> MAHHHHHHMKFAFVFPGQGSQSVGMLNAFADVAVVRETLDEASDALGQDIGKLIADGPADELNLTTNTQPVMLTAAYACYRAWQQAGGAQPSIVAGHSLGEYTALVAAGAIAFRDALPLVRFRAQAMQTAVPVGVGGMAAILGLDDDTVRAVCAEASATGVVEAVNFNAPAQVVIAGTKAGIEKACEIAKE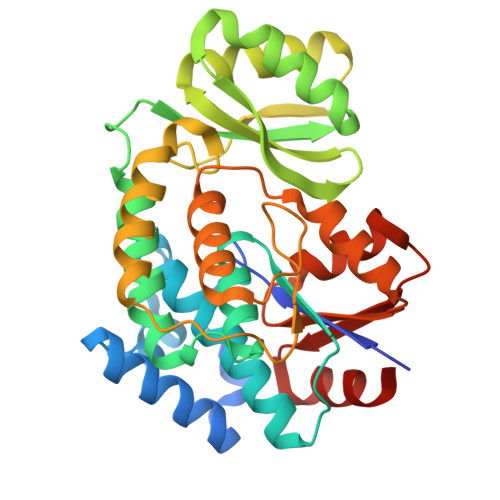KGAKRALPLPVSAPFHSSLLKPASDKLREYLAGVDVKAPKISVVNNIDVAVVSDPAAIKDALVRQAAGPVRWVECVQHIAREGVTHVIECGPGKVLAGLTKRIDGNLVGASVFDPASLDEALKLAAA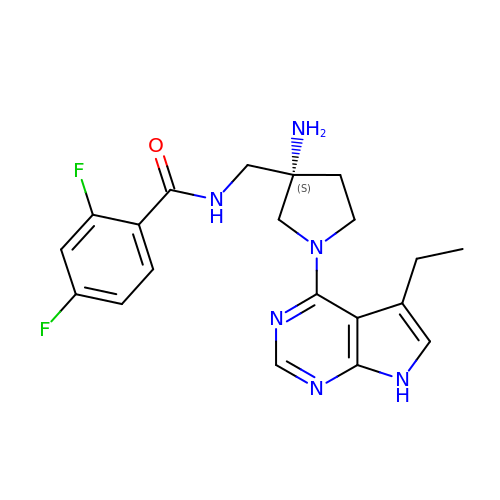N-{[(3S)-3-amino-1-(5-ethyl-7H-pyrrolo[2,3-d]pyrimidin-4-yl)pyrrolidin-3-yl]methyl}-2,4-difluorobenzamide | C20 H22 F2 N6 O | MOZRQQTUYAYCQT-FQEVSTJZSA-N> MAEVLKLHGAWPSPFSCRVIWALKLKGIPYEYVEEDLFNKSPLLLQYNPVHKKIPVLVHGGKPICESTIILEYLDETWPENPLLPSDPHERAVARFWVKFIEDKGTAIWNIFRTKGEELEKAVKNCLEVLKTIEEHAMG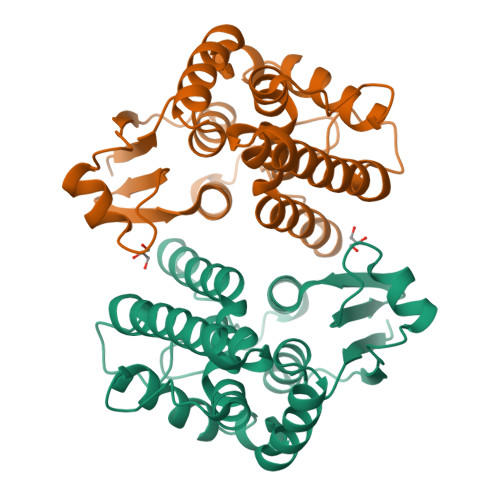VSDDKYFGGDKIGIVDIAFCGIAHWLGVIEEVAGVKVLESQKFPRLHAWTENFKEAPIIKENLPDRDQMTAFFKRRREMILASA> MATEHPEPPKAELQLPPPPPPGHYGAWAAQELQAKLAEIGAPIQGNREELVERLQSYTRQTGIVLNRPVLRGEDGDKAAPPPMSAQLPGIPMPPPPLGLPPLQPPPPPPPPPPGLGLGFPMAHPPNLGPPPPLRVGEPVALSEEERLKLAQQQAALLMQQEERAKQQGDHSLKEHELLEQQKRAAVLLEQERQQEIAKMGTPVPRPPQDMGQIGVRTPLGPRVAAPVGPVGPTPTVLPMGAPVPRPRGPPPPPGDENREMDDPSVGPKIPQALEKILQLKESRQEEMNSQQEEEEMETDARSSLGQSASETEEDTVSVSKKEKNRKRRNRKKKKKPQRVRGVSSESSGDREKDSTRSRGSDSPAADVEIEYVTEEPEIYEPNFIFFKRIFEAFKLTDDVKKEKEKEPEKLDKLENSAAPKKKGFEEEHKDSDDDSSDDEQEKKPEAPKLSKKKLRRMNRFTVAELKQLVARPDVVEMHDVTAQDPKLLVHLKATRNSVPVPRHWCFKRKYLQGKRGIEKPPFELPDFIKRTGIQEMREALQEKEEQKTMKSKMREKVRPKMGKIDIDYQKLHDAFFKWQTKPKLTIHGDLYYEGKEFETRLKEKKPGDLSDELRISLGMPVGPNAHKVPPPWLIAMQRYGPPPSYPNLKIPGLNSPIPESCSFGYHAGGWGKPPVDETGKPLYGDVFGTNAAEFQTKTEEEEIDRTPWGELEPSDEESSEEEEEEESDEDKPDETGFITPADSGLITPGGFSSVPAGMETPELIELRKKKIEEAMDGSETPQLFTVLPEKRTATVGGAMMGSTHIYDMSTVMSRKGPAPELQGVEVALAPEELELDPMAMTQKYEEHVREQQAQVEKEDFSDMVAEHAAKQKQKKRKAQPQDSRGGSKKYKEFKF;> METILEQQRRYHEEKERLMDVMAKEMLTKKSTLRDQINSDHRTRAMQDRYMEVSGNLRDLYDDKDGLRKEELNAISGPNEFAEFYNRLKQIKEFHRKHPNEICVPMSVEFEELLKARENPSEEAQNLVEFTDEEGYGRYLDLHDCYLKYINLKASEKLDYITYLSIFDQLFDIPKERKNAEYKRYLEMLLEYLQDYTD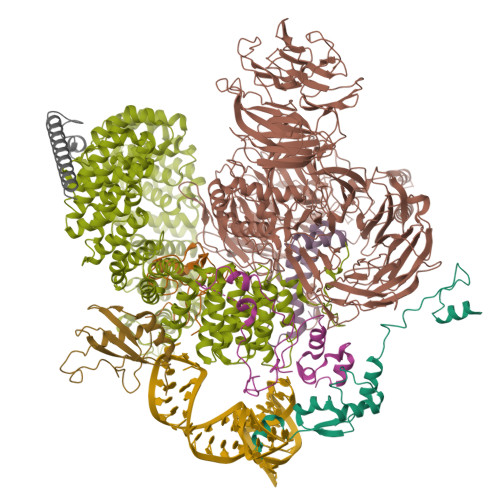RVKPLQDQNELFGKIQAEFEKKWENGTFPGWPKETSSALTHAGAHLDLSAFSSWEELASLGLDRLKSALLALGLKCGGTLEERAQRLFSTKGKSLESLDTSLFAKNPKSKGTKRDTERNKDIAFLEAQIYEYVEILGEQRHLTHENVQRKQARTGEEREEEEEEQISESESEDEENEIIYNPKNLPLGWDGKPIPYWLYKLHGLNINYNCEICGNYTYRGPKAFQRHFAEWRHAHGMRCLGIPNTAHFANVTQIEDAVSLWAKLKLQKASERWQPDTEEEYEDSSGNVVNKKTYEDLKRQGLL;> MGRESRHYRKRSASRGRSGSRSRSRSPSDKRSKRGDDRRSRSRDRDRRRERSRSRDKRRSRSRDRKRLRRSRSRERDRSRERRRSRSRDRRRSRSRSRGRRSRSSSPGNKSKKTENRSRSKEKTDGGESSKEKKKDKDDKEDEKEKDAGNFDQNKLEEEMRKRKERVEKWREEQRKKAMENIGELKKEIEEMKQGKKWSLEDDDDDEDDPAEAEKEGNEMEGEELDPLDAYMEEVKEEVKKFNMRSVKGGGGNEKKSGPTVTKVVTVVTTKKAVVDSDKKKGELMENDQDAMEYSSEEEEVDLQTALTGYQTKQRKLLEPVDHGKIEYEPFRKNFYVEVPELAKMSQEEVNVFRLEMEGITVKGKGCPKPIKSWVQCGISMKILNSLKKHGYEKPTPIQTQAIPAIMSGRDLIGIAKTGSGKTIAFLLPMFRHIMDQRSLEEGEGPIAVIMTPTRELALQITKECKKFSKTLGLRVVCVYGGTGISEQIAELKRGAEIIVCTPGRMIDMLAANSGRVTNLRRVTYVVLDEADRMFDMGFEPQVMRIVDNVRPDRQTVMFSATFPRAMEALARRILSKPIEVQVGGRSVVCSDVEQQVIVIEEEKKFLKLLELLGHYQESGSVIIFVDKQEHADGLLKDLMRASYPCMSLHGGIDQYDRDSIINDFKNGTCKLLVATSVAARGLDVKHLILVVNYSCPNHYEDYVHRAGRTGRAGNKGYAYTFITEDQARYAGDIIKALELSGTAVPPDLEKLWSDFKDQQKAEGKIIKKSSGFSGKGFKFDETEQALANERKKLQKAALGLQDSDDEDAAVDIDEQIESMFNSKKRVKDMAAPGTSSVPAPTAGNAEKLEIAKRLALRINAQKNLGIESQDVMQQATNAILRGGTILAPTVSAKTIAEQLAEKINAKLNYVPLEKQEEERQDGGQNESFKRYEEELEINDFPQTARWKVTSKEALQRISEYSEAAITIRGTYFPPGKEPKEGERKIYLAIESANELAVQKAKAEITRLIKEELIRLQNSYQPTNKGRYKVL;> MSGTNLDGNDEFDEQLRMQELYGDGKDGDTQTDAGGEPDSLGQQPTDTPYEWDLDKKAWFPKITEDFIATYQANYGFSNDGASSSTANVEDVHARTAEEPPQEKAPEPTDARKKGEKRKAESGWFHVEEDRNTNVYVSGLPPDITVDEFIQLMSKFGIIMRDPQTEEFKVKLYKDNQGNLKGDGLCCYLKRESVELALKLLDEDEIRGYKLHVEVAKFQLKGEYDASKKKKKCKDYKKKLSMQQKQLDWRPERRAGPSRMRHERVVIIKNMFHPMDFEDDPLVLNEIREDLRVECSKFGQIRKLLLFDRHPDGVASVSFRDPEEADYCIQTLDGRWFGGRQITAQAWDGTTDYQVEETSREREERLRGWEAFLNAPEANRGLRRSDSVSASERAGPSRARHFSEHPSTSKMNAQETATGMAFEEPIDEKKFEKTEDGGEFEEGASENNAKESSPEKEAEEGCPEKESEEGCPKRGFEGSCSQKESEEGNPVRGSEEDSPKKESKKKTLKNDCEENGLAKESEDDLNKESEEEVGPTKESEEDDSEKESDEDCSEKQSEDGSEREFEENGLEKDLDEEGSEKELHENVLDKELEENDSENSEFEDDGSEKVLDEEGSEREFDEDSDEKEEEEDTYEKVFDDESDEKEDEEYADEKGLEAADKKAEEGDADEKLFEESDDKEDEDADGKEVEDADEKLFEDDDSNEKLFDEEEDSSEKLFDDSDERGTLGGFGSVEEGPLSTGSSFILSSDDDDDDI;> MAKIAKTHEDIEAQIREIQGKKAALDEAQGVGLDSTGYYDQEIYGGSDSRFAGYVTSIAATELEDDDDDYSSSTSLLGQKKPGYHAPVALLNDIPQSTEQYDPFAEHRPPKIADREDEYKKHRRTMIISPERLDPFADGGKTPDPKMNARTYMDVMREQHLTKEEREIRQQLAEKAKAGELKVVNGAAASQPPSKRKRRWDQTADQTPGATPKKLSSWDQAETPGHTPSLRWDETPGRAKGSETPGATPGSKIWDPTPSHTPAGAATPGRGDTPGHATPGHGGATSSARKNRWDETPKTERDTPGHGSGWAETPRTDRGGDSIGETPTPGASKRKSRWDETPASQMGGSTPVLTPGKTPIGTPAMNMATPTPGHIMSMTPEQLQAWRWEREIDERNRPLSDEELDAMFPEGYKVLPPPAGYVPIRTPARKLTATPTPLGGMTGFHMQTEDRTMKSVNDQPSGNLPFLKPDDIQYFDKLLVDVDESTLSPEEQKERKIMKLLLKIKNGTPPMRKAALRQITDKAREFGAGPLFNQILPLLMSPTLEDQERHLLVKVIDRILYKLDDLVRPYVHKILVVIEPLLIDEDYYARVEGREIISNLAKAAGLATMISTMRPDIDNMDEYVRNTTARAFAVVASALGIPSLLPFLKAVCKSKKSWQARHTGIKIVQQIAILMGCAILPHLRSLVEIIEHGLVDEQQKVRTISALAIAALAEAATPYGIESFDSVLKPLWKGIRQHRGKGLAAFLKAIGYLIPLMDAEYANYYTREVMLILIREFQSPDEEMKKIVLKVVKQCCGTDGVEANYIKTEILPPFFKHFWQHRMALDRRNYRQLVDTTVELANKVGAAEIISRIVDDLKDEAEQYRKMVMETIEKIMGNLGAADIDHKLEEQLIDGILYAFQEQTTEDSVMLNGFGTVVNALGKRVKPYLPQICGTVLWRLNNKSAKVRQQAADLISRTAVVMKTCQEEKLMGHLGVVLYEYLGEEYPEVLGSILGALKAIVNVIGMHKMTPPIKDLLPRLTPILKNRHEKVQENCIDLVGRIADRGAEYVSAREWMRICFELLELLKAHKKAIRRATVNTFGYIAKAIGPHDVLATLLNNLKVQERQNRVCTTVAIAIVAETCSPFTVLPALMNEYRVPELNVQNGVLKSLSFLFEYIGEMGKDYIYAVTPLLEDALMDRDLVHRQTASAVVQHMSLGVYGFGCEDSLNHLLNYVWPNVFETSPHVIQAVMGALEGLRVAIGPCRMLQYCLQGLFHPARKVRDVYWKIYNSIYIGSQDALIAHYPRIYNDDKNTYIRYELDYIL;> MFLYNLTLQRATGISFAIHGNFSGTKQQEIVVSRGKILELLRPDPNTGKVHTLLTVEVFGVIRSLMAFRLTGGTKDYIVVGSDSGRIVILEYQPSKNMFEKIHQETFGKSGCRRIVPGQFLAVDPKGRAVMISAIEKQKLVYILNRDAAARLTISSPLEAHKANTLVYHVVGVDVGFENPMFACLEMDYEEADNDPTGEAAANTQQTLTFYELDLGLNHVVRKYSEPLEEHGNFLITVPGGSDGPSGVLICSENYITYKNFGDQPDIRCPIPRRRNDLDDPERGMIFVCSATHKTKSMFFFLAQTEQGDIFKITLETDEDMVTEIRLKYFDTVPVAAAMCVLKTGFLFVASEFGNHYLYQIAHLGDDDEEPEFSSAMPLEEGDTFFFQPRPLKNLVLVDELDSLSPILFCQIADLANEDTPQLYVACGRGPRSSLRVLRHGLEVSEMAVSELPGNPNAVWTVRRHIEDEFDAYIIVSFVNATLVLSIGETVEEVTDSGFLGTTPTLSCSLLGDDALVQVYPDGIRHIRADKRVNEWKTPGKKTIVKCAVNQRQVVIALTGGELVYFEMDPSGQLNEYTERKEMSADVVCMSLANVPPGEQRSRFLAVGLVDNTVRIISLDPSDCLQPLSMQALPAQPESLCIVEMGGTEKQDELGERGSIGFLYLNIGLQNGVLLRTVLDPVTGDLSDTRTRYLGSRPVKLFRVRMQGQEAVLAMSSRSWLSYSYQSRFHLTPLSYETLEFASGFASEQCPEGIVAISTNTLRILALEKLGAVFNQVAFPLQYTPRKFVIHPESNNLIIIETDHNAYTEATKAQRKQQMAEEMVEAAGEDERELAAEMAAAFLNENLPESIFGAPKAGNGQWASVIRVMNPIQGNTLDLVQLEQNEAAFSVAVCRFSNTGEDWYVLVGVAKDLILNPRSVAGGFVYTYKLVNNGEKLEFLHKTPVEEVPAAIAPFQGRVLIGVGKLLRVYDLGKKKLLRKCENKHIANYISGIQTIGHRVIVSDVQESFIWVRYKRNENQLIIFADDTYPRWVTTASLLDYDTVAGADKFGNICVVRLPPNTNDEVDEDPTGNKALWDRGLLNGASQKAEVIMNYHVGETVLSLQKTTLIPGGSESLVYTTLSGGIGILVPFTSHEDHDFFQHVEMHLRSEHPPLCGRDHLSFRSYYFPVKNVIDGDLCEQFNSMEPNKQKNVSEELDRTPPEVSKKLEDIRTRYAF;> MTDRYTIHSQLEHLQSKYIGTGHADTTKWEWLVNQHRDSYCSYMGHFDLLNYFAIAENESKARVRFNLMEKMLQPCGPPADKPEEN;> MAKHHPDLIFCRKQAGVAIGRLCEKCDGKCVICDSYVRPCTLVRICDECNYGSYQGRCVICGGPGVSDAYYCKECTIQEKDRDGCPKIVNLGSSKTDLFYERKKYGFKKR The carboxysome is a natural proteinaceous organelle for carbon fixation in cyanobacteria and chemoautotrophs. It comprises hundreds of protein homologs that self-assemble to form a polyhedral shell structure to sequester cargo enzymes, ribulose 1,5-bisphosphate carboxylase/oxygenase (Rubisco), and carbonic anhydrases. Recent studies have identified the chaperone protein CcmS, which can interact with CcmK1, facilitating β-carboxysome assembly in Syn6803. Here, we determined the structure of the chaperone protein CcmS, which has recently been identified to be involved in β-carboxysome assembly, and its interactions with β-carboxysome proteins.

To decipher how CcmS interacts with the C-terminal domain of CcmK1, we co-crystallized CcmS and the C-terminus of CcmK1 containing 15 amino acids (CcmK1-C15). After a period of crystal growth, we obtained high-quality crystals and solved the 1.67 Å crystal structure of the CcmS/CcmK1-C15 complex in space group P41212 by molecular replacement. In the refined structure, each asymmetric unit contains a CcmS dimer and a CcmK1-C15. CcmK1-C15 binds to one side of the CcmS dimer along the longitudinal direction through hydrogen bonds and salt bridges. The polar contacts between CcmK1-C15 and CcmS involve Arg101-Asp51, Arg101-Gln53, Ile107-Phe58, Asn105-Tyr60, Phe110-Asp126, Gly111-Asp126, and Arg112-Glu130 interactions. Furthermore, these amino acid residues involved in the interactions between CcmS and CcmK1-C15 are conserved, implying a general interaction manner of CcmS and CcmK1 among different cyanobacterial species. Intriguingly, superposition of the crystal structures of CcmS alone and the CcmS/CcmK1-C15 complex revealed that the binding with CcmK1-C15 resulted in conformational changes of CcmS. In particular, the α-helices in the W38-P89 region underwent a rotational shift, including the conformational change from a random curl to an α-helical structure. Additionally, the β-sheets in the I98-I103 region near CcmK1-C15 became less ordered. In the crystal structure of the CcmS/CcmK1-C15 complex, we found that one CcmK1-C15 peptide could also bind to the CcmS dimer of the neighboring asymmetric unit via Arg108-Asp51, Gly111-His57, and Arg112-Tyr60 interactions.

>[2x]SKWRSQLDRFVKENQQDLAALFWGLWLENGDSQGTIGIDLQPTPHFVYCPKDAVEKLNNNVENRLQELLGIIEHNQPEIEVLMIGIGKGEIKLIQFAPEPPPPVCFEQVGKDIDGLLELLEQRMSGEIVV;> FRENVNAIRPFGRRP>[2x]MQKAITLTHRGMTLRGMEHIPEKSLDEKVPAVILFHGFTGTKLEPHRLFLKISRALEKQGIASFRFDFLGSGESDGDFEEMTVSKEIEEAHAIVDFVKRDGRIDPSHIYLLGLSMGG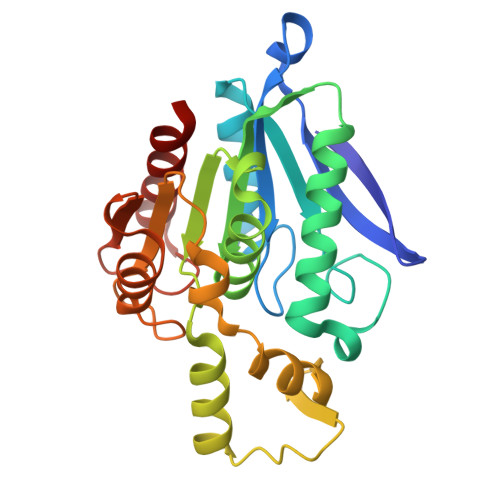LVASVVAGERPNDVAKLILMAPAGNMYELITETIRQENIDVTAPYFDHGGNLVGRSFLEDLQTINVFERAKPYDGPVLLIHGTEDDVVPHRVSHLYEQLCYGSRATVHLIEGANHTFDGHRWETEVIKTILGFVS GLYCERALDEHYDE-3-PHOSPHATE | C3 H7 O6 P | 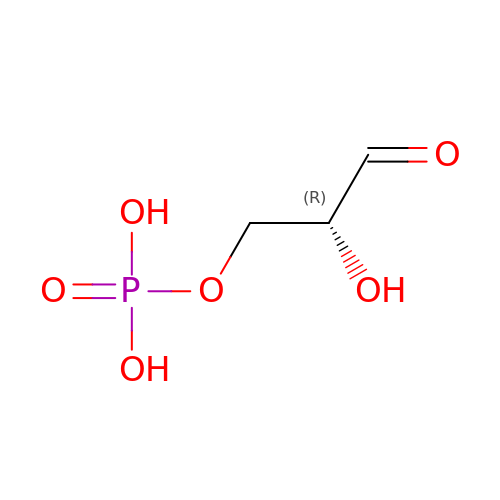LXJXRIRHZLFYRP-VKHMYHEASA-N> INFYKDSYAASASKQDFSQDPSKFTEPVADALKAG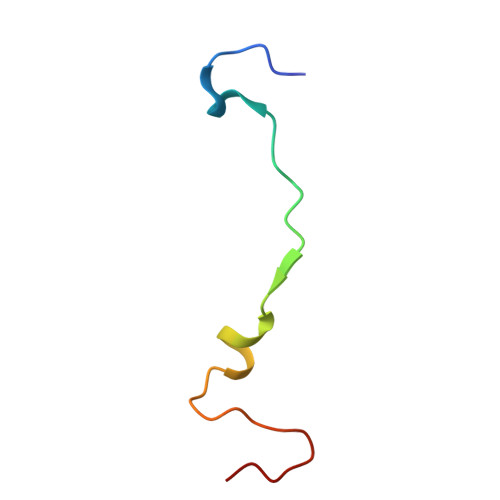APVL>[2x]GSHMTSEQFEYHLTGKEILEKEFKTGLRGYSPEDVDEFLDMVIKDYS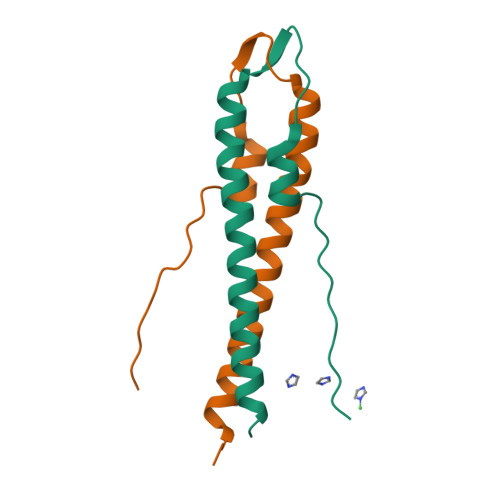TFTQEIEALQAENIRLVQELDNAPLRTST>[2x]GHMSPNYDKWEMERTDITMKHKLGGGQYGEVYEGVWKKYSLTVAVKTLKEDTMEVEEFLKEAAVMKEIKHPNLVQLLGVCTREPPFYIITEFMTYGNLLDYLRECNRQEVNA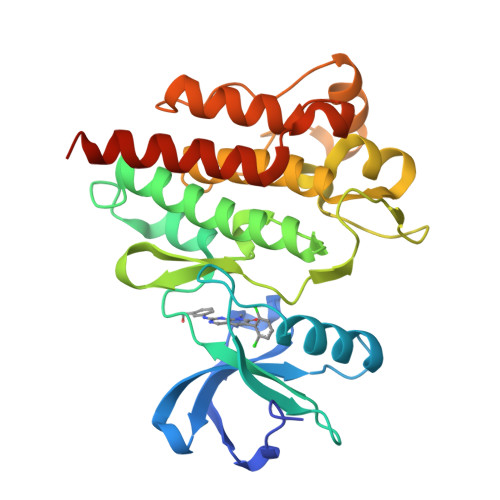VVLLYMATQISSAMEYLEKKNFIHRDLAARNCLVGENHLVKVADFGLSRLMTGDTYTAPAGAKFPIKWTAPESLAYNKFSIKSDVWAFGVLLWEIATYGMSPYPGIDLSQVYELLEKDYRMERPEGCPEKVYELMRACWQWNPSDRPSFAEIHQAFETMFQESSISDEVEKELGK> DII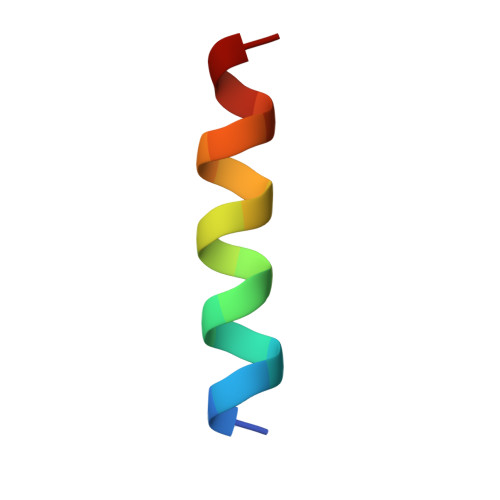RNIARHLAQVGDSMD> MPKTISVRVTTMDAELEFAIQPNTTGKQLFDQVVKTIGLREVWFFGLQYQDTKGFSTWLKLNKKVTAQDVRKESPLLFKFRAKFYPEDVSEELIQDITQRLFFLQVKEGILNDDIYCPPETAVLLASYAVQSKYGDFNKEVHKSGYLAGDKLLPQRVLEQHKLNKDQWEERIQVWHEEHRGMLREDAVLEYLKIAQDLEMYGVNYFSIKNKKGSELWLGVDALGLNIYEQNDRLTPKIGFPWSEIRNISFNDKKFVIKPIDKKAPDFV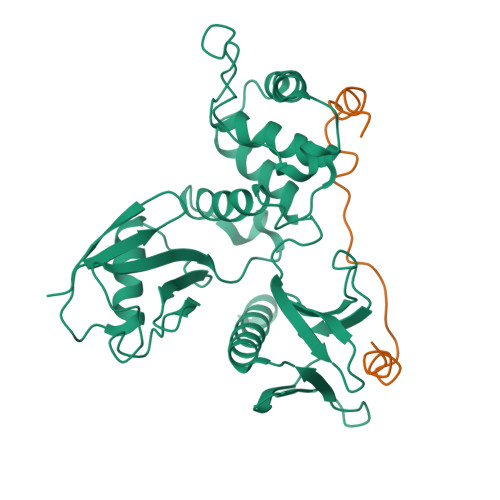FYAPRLRINKRILALCMGNHELYMRRRKP;> CLDFNISLAMAKERAHQKRSSKRAPQMDWSKKNELFSNL> VFHKIRNEDLIFNESLGQGTFTKIFKGVRREVGDYGQLHETEVLLKVLDKAHRNYSESFFEAASMMSKLSHKHLVLNYGVCFCGDENILVQEFVKFGSLDTYLKKNKNCINILWKLEVAKQLAAAMHFLEENTLIHGNVCAKNILLIREEDRKTGNPPFIKLSDPGISITVLPKDILQERIPWVPPECIENPKNLNLATDKWSFGTTLWEICSGGDKPLSALDSQRKLQFYEDRHQLPAPKAAELANLINNCMDYEPDHRPSFRAIIRDLNSLFTPDLVPRGSHHHHHH

JAK2, like other JAK family members, comprises a catalytically active C-terminal tyrosine kinase domain (JH1), a regulatory pseudokinase domain (JH2), and a Src homology-2 (SH2)-like domain that, together with the N-terminal FERM (N-terminal 4.1, ezrin, radixin, moesin) domain, forms the major receptor interaction moiety. The JH2 domain has a key role in mediating both negative and positive regulation of JAK kinase activity and numerous disease mutations locate in JH2, including the prevalent hyperactivating JAK2 V617F in MPN. Previous studies have demonstrated that JAK2 JH2 binds ATP and possesses regulatory autophosphorylation activity on Ser523 and Tyr570. To gain insights on the compound binding modes to JAK2 JH2 and to analyze whether any differences could be observed between binding to WT and V617F, we determined the crystal structures of selected small molecules with JAK2 JH2 WT and V617F.

Four hits, i.e., diaminotriazole compounds 1 and Cdk1/2 inhibitor III, and aminopurine analogs Cdk2 inhibitor IV and 7 bound JAK2 JH2 (V617F and wt) and JH1 domains with IC50 values at or below lower detection limit of assay (3.5 µM). Since the compound binding does not induce significant changes in the ATP pocket, we compared the regions around residue 617 and the helix Cα between WT and V617F structures. It has been noted before that compound binding to JAK2 JH2 V617F can disrupt the aromatic packing of F617-F595-F594 and the conformation of F595 and F594 can be reverted back to the JAK2 JH2 WT conformation. In structures complexed with 6, 36, and 16, a WT-like conformation for the phenylalanines was observed. However, the Gln626-Leu624 switch is not present in the complex with 6 but the structure still assumes a WT-like Phe594-Phe595 conformation. Interestingly, the packing of F617 against F595 observed in the V617F-ATP complex was not evident in any of our structures and the residue often displayed poor electron density suggesting high flexibility.> MKPPQQQHEAFPLFKGATRLPTIWGVPMIPLMAMVMGVAVIALTVSIWWWALVP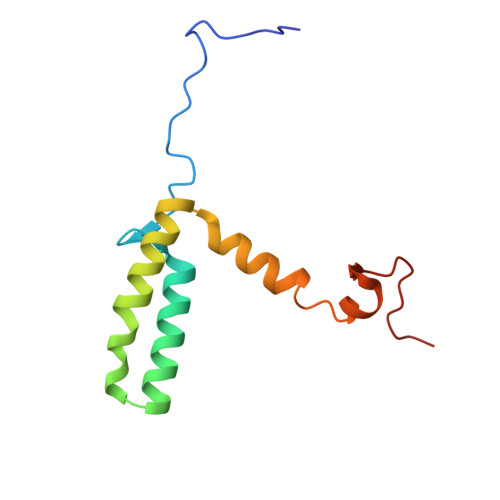PLWFIMAQITKNDDKAFRIWWLWIDTKFRNRNKGFWGASSYSPANYRKRR> TYGIRLRVWGDYACFTRPEMKVERVSYDVMPPSAARGILEAIHWKPAIRWIVDRIHVLRPIVFDNVRRNEVSSKIPKPNPATAMRDRKPLYFLVDDGSNRQQRAATLLRNVDYVIE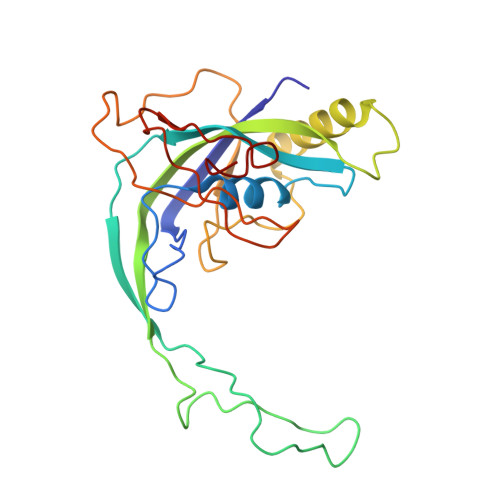AHFELTDKAGAEDNAGKHLDIFRRRARAGQSFQQPCLGCREFPASFELLEGDVPLSCYAGEKRDLGYMLLDIDFERDMTPLFFKAVMEDGVITPPSRTSPEVRA> MEPHSLRYNLMVLSQDGSVQSGFLAEGHLDGQPFLRYDRQKRRAKPQGQWAEDVLGAETWDTETEDLTENGQDLRRTLTHIKDQKGGLHSLQEIRVCEIHEDSSTRGSRHFYYNGELFLSQNLETQESTVPQSSRAQTLAMNVTNFWKEDAMKTKTHYRAMQADC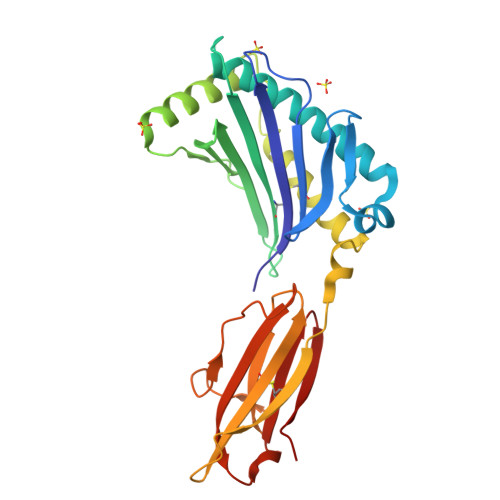LQKLQRYLKSGVAIRRTVPPMVNVTCSEVSEGNITVTCRASSFYPRNITLTWRQDGVSLSHNTQQWGDVLPDGNGTYQTWVATRIRQGEEQRFTCYMEHSGNHGTHPVPS> MKVVVQIKDFDKVPQ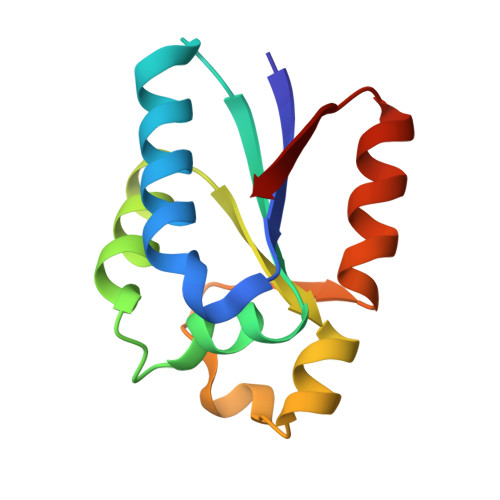ALQSVLNLFLDLGNAEIEVVLHQSAIKALLLNSPTRSIIEELIKLNILIVGCEHSIRSQNLDHRQLIDGIKIVRSGVGEIVRKQSEGWIYLAL Trans-nonachlor 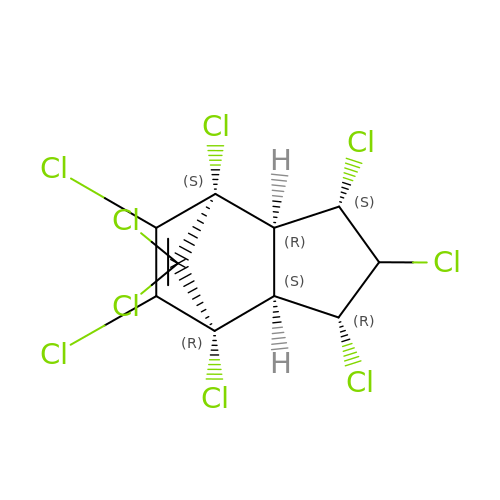| C10 H5 Cl9 | OCHOKXCPKDPNQU-DFACZZRHSA-N>RLSLQNTAEIQHCLVNAGDVGCGVFECFENNSCEIRGLHGICMTFLHNAGKFDAQGKSFIKDALKCKAHALRHRFGCISRKCPAIREMVSQLQRECYLKHDLCAAAQENTRVIVEMIHFKDLLLHEPYVDLVNLLLTCGEEVKEAITHSVQVQCEQNWGSLCSILSFC[2x];>EARGATEEPSPPSRALYFSGRGEQLRLRADLELPRDAFTLQVWLRAEGGQRSPAVITGLYDKCSYISRDRGWVVGIHTISDQDNKDPRYFFSLKTDRARQVTTINAHRSYLPGQWVYLAATYDGQFMKLYVNGAQVATSGEQVGGIFSPLTQKCKVLMLGGSALNHNYRGYIEHFSLWKVARTQREILSDMETHGAHTALPQLLLQENWDNVKHAWSPMKDGSSPKVEFSNAHGFLLDTSLEPPLCGQTLCDNTEVIASYNQLSSFRQPKVVRYRVVNLYEDDHKNPTVTREQVDFQHHQLAEAFKQYNISWELDVLEVSNSSLRRRLILANCDISKIGDENCDPECNHTLTGHDGGDCRHLRHPAFVKKQHNGVCDMDCNYERFNFDGGECCDPEITNVTQTCFDPDSPHRAYLDVNELKNILKLDGSTHLNIFFAKSSEEELAGVATWPWDKEALMHLGGIVLNPSFYGMPGHTHTMIHQIGHSLGLYHVFRGISEIQSCSDPCMETEPSFETGDLCNDTNPAPKHKSCGDPGPGNDTCGFHSFFNTPYNNFMSYADDDCTDSFTPNQVARMHCYLDLVYQGWQPSRKPAPVALAPQVLGHTTDSVTLEWFPPIDGHFFERELGSACHLCLEGRILVQYASNASSPMPCSPSGHWSPREAEGHPDVEQPCKSSVRTWSPNSAVNPHTVPPACPEPQGCYLELEFLYPLVPESLTIWVTFVSTDWDSSGAVNDIKLLAVSGKNISLGPQNVFCDVPLTIRLWDVGEEVYGIQIYTLDEHLEIDAAMLTSTADTPLCLQCKPLKYKVVRDPPLQMDVASILHLNRKFVDMDLNLGSVYQYWVITISGTEESEPSPAVTYIHGSGYCGDGIIQKDQGEQCDDMNKINGDGCSLFCRQEVSFNCIDEPSRCYFHDGDGVCEEFEQKTSIKDCGVYTPQGFLDQWASNASVSHQDQQCPGWVIIGQPAASQVCRTKVIDLSEGISQHAWYPCTISYPYSQLAQTTFWLRAYFSQPMVAAAVIVHLVTDGTYYGDQKQETISVQLLDTKDQSHDLGLHVLSCRNNPLIIPVVHDLSQPFYHSQAVRVSFSSPLVAISGVALRSFDNFDPVTLSSCQRGETYSPAEQSCVHFACEKTDCPELAVENASLNCSSSDRYHGAQCTVSCRTGYVLQIRRD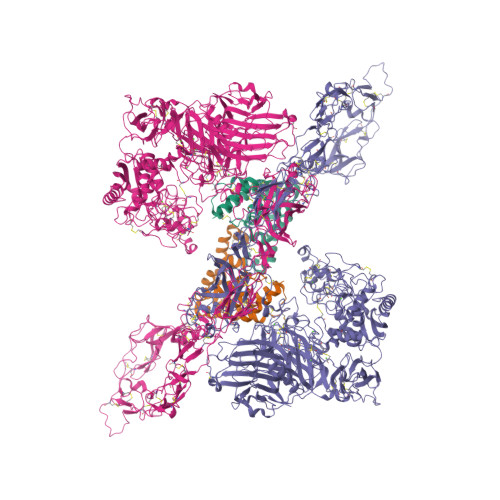DELIKSQTGPSVTVTCTEGKWNKQVACEPVDCSIPDHHQVYAASFSCPEGTTFGSQCSFQCRHPAQLKGNNSLLTCMEDGLWSFPEALCELMCLAPPPVPNADLQTARCRENKHKVGSFCKYKCKPGYHVPGSSRKSKKRAFKTQCTQDGSWQEGACVPVTCDPPPPKFHGLYQCTNGFQFNSECRIKCEDSDASQGLGSNVIHCRKDGTWNGSFHVCQEMQGQCSVPNELNSNLKLQCPDGYAIGSECATSCLDHNSESIILPMNVTVRDIPHWLNPTRVERVVCTAGLKWYPHPALIHCVKGCEPFMGDNYCDAINNRAFCNYDGGDCCTSTVKTKKVTPFPMSCDLQGDCACRDPQAQEHS[2x]Cystathionine beta-synthase (CBS) is an essential metabolic enzyme across all domains of life for the production of glutathione, cysteine, and hydrogen sulfide. Human CBS adopts a unique multi-domain structure: an N-terminal haem binding domain (residues 38–74), a central PLP-dependent catalytic domain (CD, residues 75–382), and a C-terminal regulatory domain (RD, residues 411–551)5,11,12. The RD adopts the evolutionarily conserved Bateman module, consisting of two tandem CBS motifs (CBS-1 and CBS-2) and a surface-exposed loop (residues 516–525) extending from a CBS-2 motif. Here we show using cryo-electron microscopy that full-length human CBS in the basal and SAM-bound activated states polymerises as filaments mediated by a conserved regulatory domain loop.

Though both full-length CBS constructs resulted in highly similar filament maps, one key difference was the observed protein degradation and the presence of slightly shorter oligomers of the CBSFL construct without a permanent His-tag. Consequently, along with the filament classes, we observed 2D averages of this construct that represented these degradation products. Another collection of classes resulted in a 3.8 Å map of a degraded CBS tetramer. Here two degraded heterodimers, composed of one full-length protomer and one RD-degraded catalytic domain protomer, interact through a single Bateman–Bateman interface, highly like the arrangement seen in the intact filament. The degradation of the RD renders the active site loops within the catalytic domain of the full-length CBS in a more opened state. It is unknown if this degradation is due to recombinant expression or is related to a biological function of CBS. Due to this heterogeneity, the reported tetrameric state of CBS is likely to be two dimers interacting through a single Bateman module pair but additionally could also be formed via the degradation of the Bateman module that we have shown here.

>[4x]SMPSETPQAEVGPTGCPHRSGPHSAKGSLEKGSPEDKEAKEPLWIRPDAPSRCTWQLGRPASESPHHHTAPAKSPKILPDILKKIGDTPMVRINKIGKKFGLKCELLAKCEFFNAGGSVKDRISLRMIEDAERDGTLKPGDTIIEPTSGNTGIGLALAAAVRGYRCIIVMPEKMSSEKVDVLRALGAEIVRTPTNARFDSPESHVGVAWRLKNEIPNSHILDQYRNASNPLAHYDTTADEILQQCDGKLDMLVASVGTGGTITGIARKLKEKCPGCRIIGVDPEGSILAEPEELNQTEQTTYEVEGIGYDFIPTVLDRTVVDKWFKSNDEEAFTFARMLIAQEGLLCGGSAGSTVAVAVKAAQELQEGQRCVVILPDSVRNYMTKFLSDRWMLQKGFLKEEDLTEKKPWWWHLRVQELGLSAPLTVLPTITCGHTIEILREKGFDQAPVVDEAGVILGMVTLGNMLSSLLAGKVQPSDQVGKVIYKQFKQIRLTDTLGRLSHILEMDHFALVVHEQIQYHSTGKSSQRQMVFGVVTAIDLLNFVAAQERDQK>MTLSGRIPLGGQVTDLGYAAGWRLVRAMPEAMAQGVFGAGARYAARNGGPEQLRRNLARVVGKPPADVPDDLIRASLASYARYWREAFRLPAMDHGRLGEQLDVIDIDHLWSALDAGRGAVLALPHSGNWDMAGVWLVQNYGPFTTVAERLKPESLYRRFVEYRESLGFEVLPLTGGERPPFEVLAERLTDNRPICLMAERDLTRSGVQVDFFGEATRMPAGPAKLAIETGAALFPVHCWFEGDGWGMRVYPELDTSSGDVT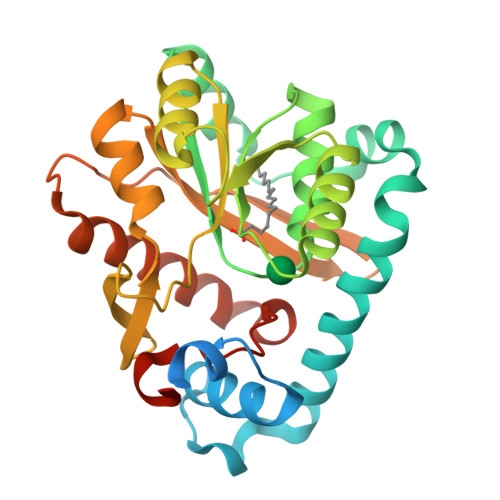AITQALADRFAANIATYPADWHMLQPQWIADLSDERRARLGT[4x]Here, we report the isolation of a novel protein from Methylomonas sp. expected to be a putative enzyme based on sequence similarity to ketose 3‐epimerase. The synthesized gene encoding the deduced ketose 3‐epimerase was expressed as a recombinant enzyme in Escherichia coli, and it exhibited the highest enzymatic activity toward l‐ribulose, followed by d‐ribulose and d‐allulose. The X‐ray structure analysis of l‐ribulose 3‐epimerase from Methylomonas sp. (MetLRE) revealed a homodimeric enzyme, the first reported structure of dimeric l‐ribulose 3‐epimerase.

d‐Allulose has potential as a low‐calorie sweetener which can suppress fat accumulation. MetLRE is the first dimeric l‐ribulose 3‐epimerase identified to exhibit high relative activity toward d‐allulose.

>MAFPKRLEYGGHALVWSGDWSAAGARKAIAGAARAGYDYIEIALLDPWQIDVALTKDLLQEYNLRAHASLGLSAATDVTSTDPAIVAKGDELLRKATDVLYALGGSELCGVIYCALGKYPGPASRENRANSVAAMQRLADYAADKGINIDLEVVNRYETNIMNTGLEGLAFLDEVNRPNAFLHLDTYHMNIEENGMAKSVLAAGDRLGYVHIGESHRGYLGTGNVDFASFFAALKQIDYRGPITFESFSSEIVDPKLSNTLCVWRNLWHDSDDLAGKALEFIKQRYGSHHHHHH[2x]>MTKQHAFTREDLLRCSRGELFGPGNAQLPAPNMLMIDRIVHISDVGGKYGKGELVAELDINPDLWFFACHFEGDPVMPGCLGLDAMWQLVGFYLGWQGNPGRGRALGSGEVKFFGQVLPTAKKVTYNIHIKRT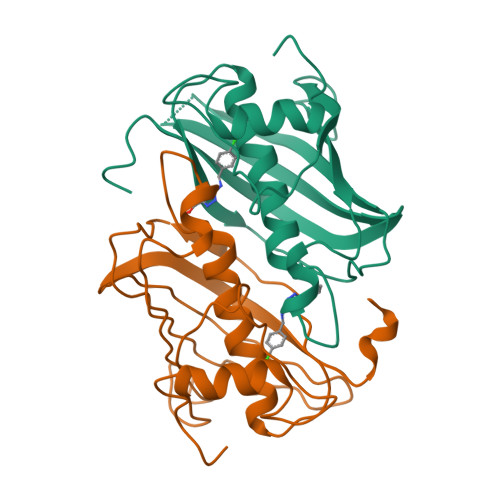INRSLVLAIADGTVSVDGREIYSAEGLRVGLFTSTDSF[5x]> GTMGVNAVHWFRKGLRL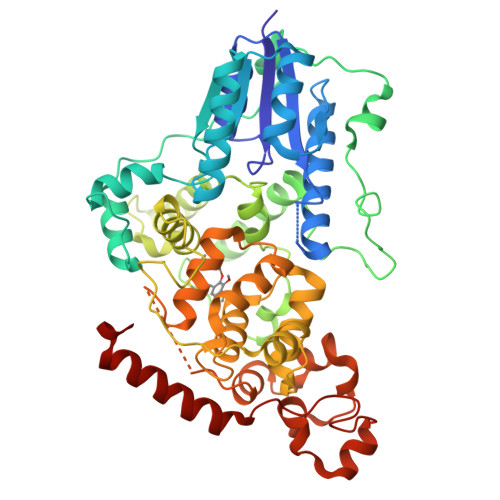HDNPALKECIQGADTIRCVYILDPWFAGSSNVGINRWRFLLQCLEDLDANLRKLNSRLFVIRGQPADVFPRLFKEWNITKLSIEYDSEPFGKERDAAIKKLATEAGVEVIVRISHTLYDLDKIIELNGGQPPLTYKRFQTLVSKMEPLEMPADTITSDVIGKCMTPLSDDHDEKYGVPSLEELGFDTDGLSSAVWPGGETEALTRLERHLERKAWVANFERPRMNANSLLASPTGLSPYLRFGCLSCRLFYFKLTDLYKKVKKNSSPPLSLYGQLLWREFFYTAATNNPRFDKMEGNPICVQIPWDKNPEALAKWAEGRTGFPWIDAIMTQLRQEGWIHHLARHAVACFLTRGDLWISWEEGMKVFEELLLDADWSINAGSWMWLSCSSFFQQFFHCYCPVGFGRRTDPNGDYIRRYLPVLRGFPAKYIYDPWNAPEGIQKVAKCLIGVNYPKPMVNHAEASRLNIERMKQIYQQLSRYRG[({[2-chloro-4-(1H-tetrazol-5-yl)phenyl]sulfonyl}amino)methyl]boronic acid | C8 H9 B Cl N5 O4 S | 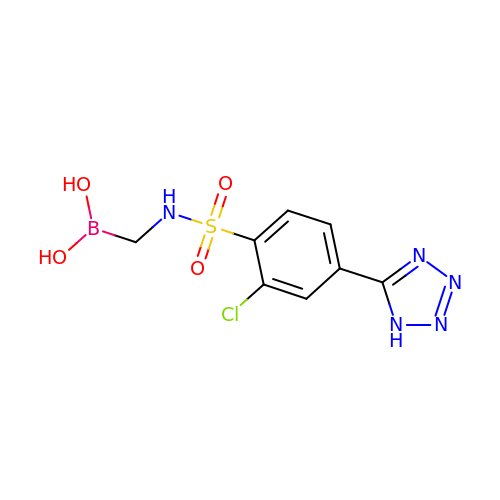NTFXGXIWMYOTKN-UHFFFAOYSA-N> LFTVTAPKEVYTVD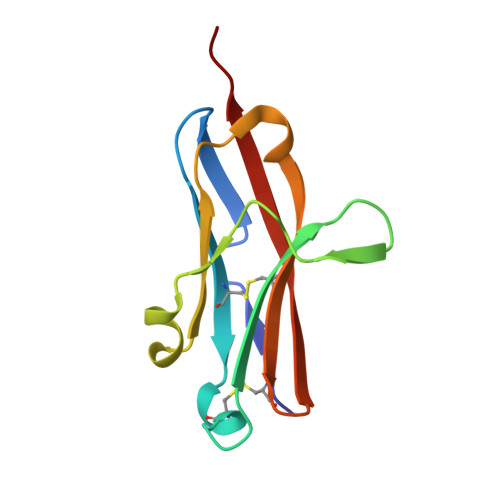VGSSVSLECDFDRRECTELEGIRASLQKVENDTSLQSERATLLEEQLPLGKALFHIPSVQVRDSGQYRCLVICGAAWDYKYLTVKVKASY>[2x]MPTLLRVYIDGPHGMGKTTTTQLLVALGSRDDIVYVPEPMTYWRVLGASETIANIYTTQHRLDQGEISAGDAAVVMTSAQITMGMPYAVTDAVLAPHIGGEAGSSHAPPPALTLIFDRHPIAALLCYPAARYLMGSMTPQAVLAFVALIPPTLPGTNIVLGALPEDRHIDRLA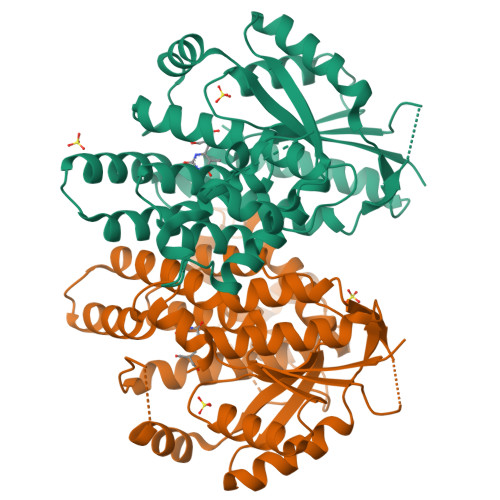KRQRPGERLDLAMLAAIRRVYGLLANTVRYLQCGGSWREDWGQLSGTAVPPQGAEPQSNAGPRPHIGDTLFTLFRAPELLAPNGDLYNVFAWALDVLAKRLRSMHVFILDYDQSPAGCRDALLQLTSGMVQTHVTTPGSIPTICDLARTFAREMGEAN> NILLQDPFAVLKEHPEKLTHTIENPLRTECLQFSPCGDYLALGCANGALVIYDMDTFRPICVPGNMLGAHVRPITSIAWSPDGRLLLTSSRDWSIKLWDLSKPSKPLKEIRFDSPIWGCQWLDAKRRLCVATIFEESDAYVIDFSNDPVASLLSKSDEKQLSSTPDHGYVLVCTVHTKHPNIIIVGTSKGWLDFYKFHSLYQTECIHSLKITSSNIKHLIVSQNGERLAINCSDRTIRQYEISIDDENSAVELTLEHKYQDVINKLQWNCILFSNNTAEYLVASTHGSSAHELYIWETTSGTLVRVLEGAEEELIDINWD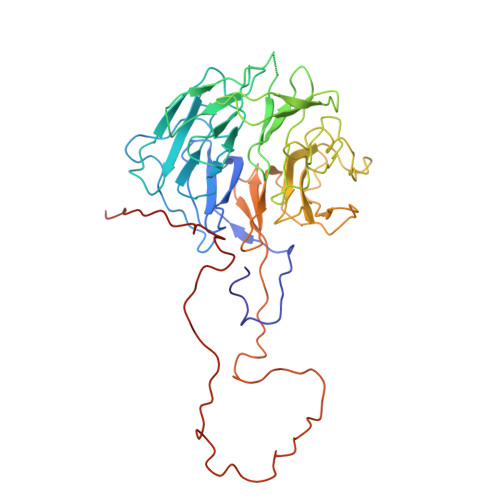FYSMSIVSNGFESGNVYVWSVVIPPKWSALAPDFEEVEENVDYLEKEDEFDEVDEAEQQQGLEQEEEIAIDLRTREQYDVRGNNLLVERFTI> MVTKVLLVSLALFALGTCQVAVNLCTQYGWPNGNYPDPYDCRKYISCNGAVATVMSCALGTVFNPNTRNCDAYGNVPICQYALPSPIVVTNICNQYGWGNGNFYHPYNCAEYIGCANGLTTVNACGAGQYYDQALGRCALAGTGYCRQYVFTPPPAPVVYPDGFDTYCSANNLATGIHPDPYSCFSYVECTFGRTTHMPCPAGLSFDRSLLVCDGNRYQNCGGNVLVGK

Brown algae utilize phlorotannin as their chemical defense against the predator Aplysia kurodai, which uses β-glucosidase (akuBGL) to digest the laminarin in algae into glucose. Moreover, A. kurodai employs Eisenia hydrolysis-enhancing protein (EHEP) as an offense to protect akuBGL activity from phlorotannin inhibition by precipitating phlorotannin. To underpin the molecular mechanism of this digestive–defensive–offensive system, we determined the structures of the apo and tannic acid (TNA, a phlorotannin analog) bound forms of EHEP, as well as the apo akuBGL. Combining docking analysis, we propose the mechanisms by which phlorotannin inhibits akuBGL by occupying the substrate-binding pocket, and EHEP protects akuBGL against this inhibition by binding with phlorotannin to free the akuBGL pocket.

Considering the lack of known homologous proteins of EHEP, we determined the structure of EHEP using the native-SAD method at a resolution of 1.15 Å, with an Rwork and Rfree of 0.18 and 0.19, respectively. The residues A21–V227 in purified EHEP (1–20 aa were cleaved during maturation) were built, whereas two C-terminal residues were disordered. The structure of EHEP consists of three PADs: PAD1 (N24–C79), PAD2 (I92–C146), and PAD3 (F164–C221), which are linked by two long loops, LL1 (Q80–N91) and LL2 (R147– G163), and arranged in a triangular shape. These three PADs share a similar structure, with a root-mean-squared difference (RMSD) of 1.065 Å over 46 Cα atoms and only ~20.3% sequence identity. The three PADs share a canonical CBM14 fold consisting of two β-sheets containing three N-terminal and two C-terminal antiparallel β-strands. Additionally, two small α-helices were appended to the N- and C-terminus in PAD1 and PAD3 but not in PAD2. The CNo1X15CNo2X5CNo3X9CNo4X12CNo5X5–9CNo6 motif (superscripts and subscripts indicate the cysteine number and number of residues between adjacent cysteines, respectively) in each PAD of EHEP formed three disulfide bonds between the following pairs: CNo1–CNo3, CNo2–CNo6, and CNo4–CNo5. Such rich disulfide bonds may play a folding role in the structural formation of EHEP, with >70% of the backbone in a loop conformation. The three PADs of EHEP are arranged in a triangular shape, forming a large cavity on the surface at the triangle center to provide a ligand-binding site.>[2x]VYLDRKLLTLEDKE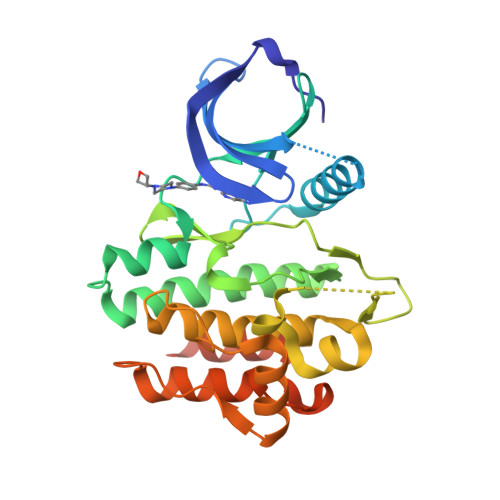LGSGNFGTVKKGYYQMKKVVKTVAVKILKNEANDPALKDELLAEANVMQQLDNPYIVRMIGICEAESWMLVMEMAELGPLNKYLQQNRHVKDKNIIELVHQVSMGMKYLEESNFVHRDLAARNVLLVTQHYAKISDFGLSKALRADENYYKAQTHGKWPVKWYAPECINYYKFSSKSDVWSFGVLMWEAFSYGQKPYRGMKGSEVTAMLEKGERMGCPAGCPREMYDLMNLCWTYDVENRPGFAAVELRLRNYYYDVVNEGHHHHHH>[8x]GAG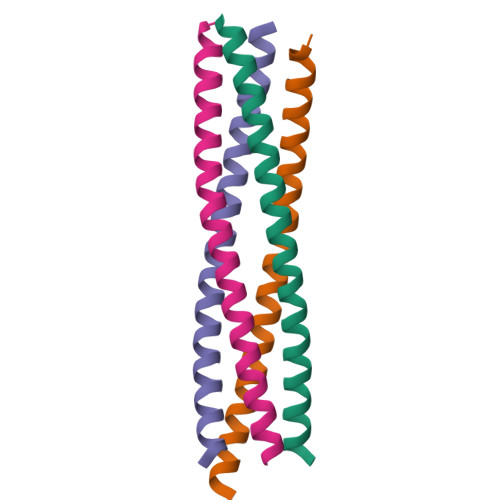SRVTFERVEQMSIQIKEVGDRVNYIKRSLQSLDSQIGHLQDLSALTVDTLKTL> KKKEEEDDDMKELEN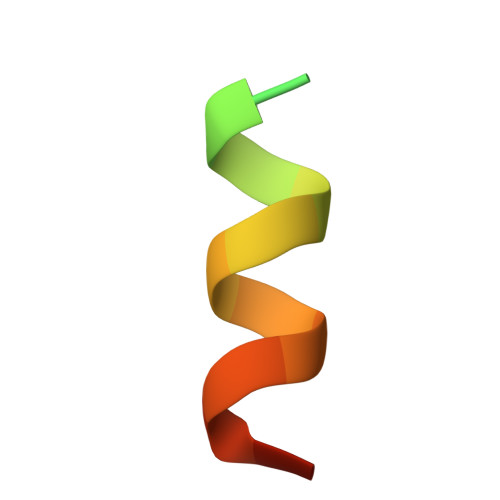WAGSM Another unicellular pappalysin is the T. forsythia KLIKK MP mirolysin, which protects the bacterium against complement-mediated bactericidal activity. It is secreted as a 66 kDa zymogen (see UniProt code A0A0F7IPS1), which when activated cleaves several physiologically relevant host proteins such as fibronectin; fibrinogen; complement proteins C3, C4 and C5; as well as antimicrobial peptide LL-37. As part of its virulence factor armamentarium, at the site of colonization it secretes mirolysin, a metallopeptidase of the unicellular pappalysin family, as a zymogen that is proteolytically auto-activated extracellularly at the Ser54–Arg55 bond. The catalytic domain conforms to the metzincin clan of metallopeptidases and contains a double calcium site, which acts as a calcium switch for activity.

A variant, in which the general base/acid Glu225 was replaced with alanine (E225A), lacked activity. This variant was used to obtain the intact zymogen for structural studies. Previously, this strategy has proven successful for other MP zymogens. We obtained two different crystal forms for native and selenomethionine-derivatized promirolysin E225A, which contained one and two protomers per asymmetric unit and diffracted to resolutions of 1.4 and 1.6 Å, respectively. The only significant deviation was observed for segment Lys51–Arg55, which contained the final activation cleavage point (Ser54–Arg55) and was flexible. Promirolysin E225A has a compact structure of approximate dimensions 60 × 45 × 45 Å, and it splits into an N-terminal 34-residue PS (Arg21–Ser54) and a downstream 274-residue metzincin-type CD (Arg55–Leu328). Tyrosine-switch Tyr286 pinches the extended segment I together with the upper-rim-strand segment Leu181–Tyr183 of the CD. In the capital interaction for latency, downstream Cys23 Sγ binds the catalytic zinc at 2.11–2.22 Å in the different structures, which is closer than typical Zn–S distances (2.31 Å), and contributes together with the three histidine ligands to a tetrahedral zinc coordination sphere [Figs. 2(c) and 2(d)]. Activation does not lead to substantial re­arrangement, i.e. the CD and the active site are already preformed in the zymogen and just shielded by the PS. Thus, the results herein indicate that latency for promirolysin and uni­cellular pappalysins probably operates based on a cysteine switch featuring a cysteine imbedded here in a conserved cysteine–glycine motif.

>GPQRTCGSELNMEQIRRTEPLKYQRITDWENQIKLHSRSVPSSTILIPVVVHVVYNNSAQNISDAQIISQIQVLNEDFRRMNADQANTPSAFANLAGNANIEFKLARRDPNGNTTNGITRTSTSTETFSMEMDNVKFSNLGGNNAWNTRRYLNIWVCNLGDDLLGYAQFPFEFQTKPNTDGVVIHYKHFGRDGSAESPYDKGRTATHAVGHWLDLRHIWGDDGGSCSGTDNIADTPNQGGYNEGCPSFPKTDHCTNTSPGVMFMNYMDYTYDACMNLFTKGQVERMRSLFDTQTGIRREMQIYANELTNPLSFS[2x]>MEIKTTTTLHRVVEETTKPLGATLVVETDISRKDVNGLARGHLVDGIPLCTPSFYADIAMQVGQYSMQRLRAGHPGAGAIDGLVDVSDMVVDKALVPHGKGPQLLRTTLTMEWPPKAAATTRSAKVKFATYFADGKLDTEHASCTVRFTSDAQLKSLRRSVSEYKTHIRQLHDGHAKGQFMRYNRKTGYKLMSSMARFNPDYMLLDYLVLNEAENEAASGVDFSLGSSEGTFAAHPAHVDAITQVAGFAMNANDNVDIEKQVYVNHGWDSFQIYQPLDNSKSYQVY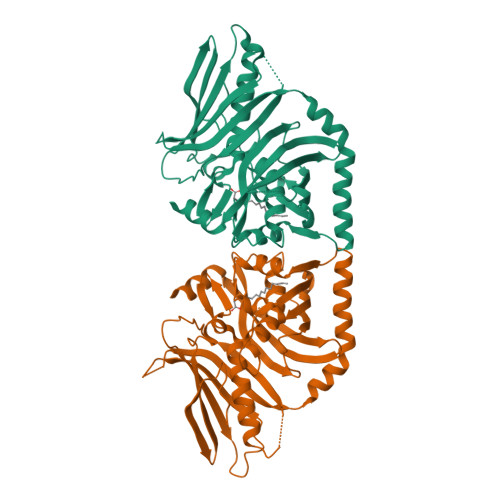TKMGQAKENDLVHGDVVVLDGEQIVAFFRGLTLRSVPRGALRVVLQTTVKKADRQLGFKTMPSPPPPTTTM[2x]> MNGIHDTGGAHGYGPVYREPNEPVFRYDWEKTVMSLLPALLANGNFNLDEFRHSIERMGPAHYLEGTYYEHWLHVFENLLVEKGVLTATEVATGKAASGKTATPVLTPAIVDGLLSTGASAAREEGARARFAVGDKVRVLNKNP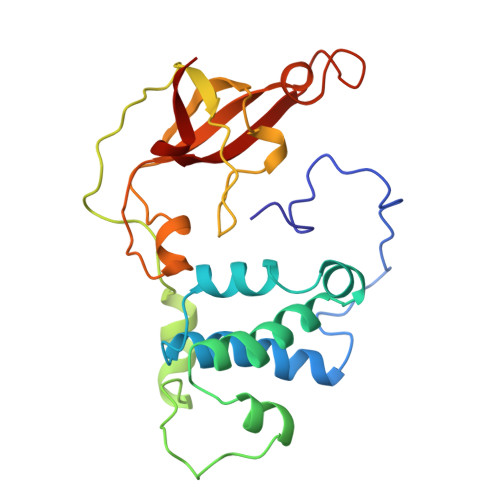VGHTRMPRYTRGKVGTVVIDHGVFVTPDTAAHGKGEHPQHVYTVSFTSVELWGQDASSPKDTIRVDLWDDYLEPA> MMSFQKIYSPTQLANAMKLVRQQNGWTQSELAKKIGIKQATISNFENNPDNTTLTTFFKILQSLELSM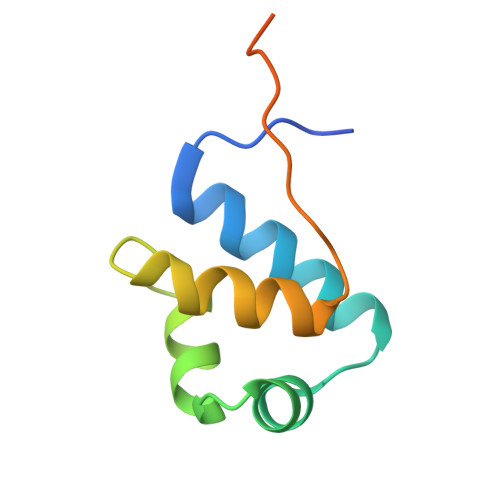TLCDAKNASPESTEQQNLEW N-[4-(2,4-difluorophenoxy)-3-(1-methyl-7-oxo-6,7-dihydro-1H-pyrrolo[2,3-c]pyridin-3-yl)phenyl]ethanesulfonamide 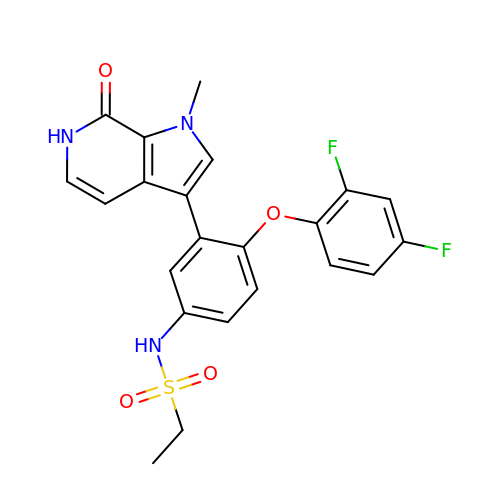| C22 H19 F2 N3 O4 S | RWDOZZPKEZJESZ-UHFFFAOYSA-N> GSHMDHLPMPKFGPLAGLRVVFSGIEIAGPFAGQMFAEWGAEVIWIENVAWADTIRVQPNYPQLSRRNLHALSLNIFKDEGREAFLKLMETTDIFIEASKGPAFARRGITDEVLWQHNPKLVIAHLSGFGQYGTEEYTNLPAYNTIAQAFSGYLIQNGDVDQPMPAFPYTAAYFSGLTATTAALAALHKVRETGKGESIDIAMYEV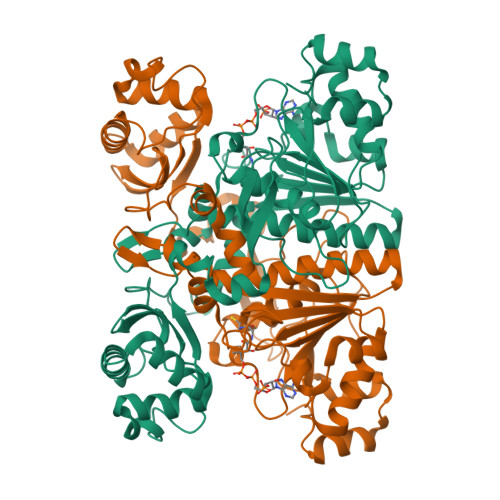MLRMGQYFMMDYFNGGEMCPRMSKGKDPYYAGCGLYKCADGYIVMELVGITQIEECFKDIGLAHLLGTPEIPEGTQLIHRIECPYGPLVEEKLDAWLATHTIAEVKERFAELNIACAKVLTVPELESNPQYVARESITQWQTMDGRTCKGPNIMPKFKNNPGQIWRGMPSHGMDTAAILKNIGYSENDIQELVSKGLAKVED> MGSSHHHHHHSSGLVPRGSHMASISKDFTNLLNTLIDGQIGAASRQTEWFNMSPDERTDYIKQVDERLQEMQQSTLSVLAAQHFQMQDNPVSVGDQLQTLQKRRQQMTDVPGTPAINAYKQQLDRDILLYRRQQTAMTHFDSTWRKVLVMLGPDDSKPLNATTLRENAVDKQAKLDTEIKRLEQQLTIQVADSTFSQKYVTLFSELQAYKDVNARYNALLKASATEEAAALGALTKVPQASDDLPVNISLLMMEERPGYIRMNVALVNASTDGRFKDFFLENGRLVVLTDGVLNFSFGTAARSLAWQQQYRLKSEPPSFRSPTYTPIRSVLVKTEFVEKYFANYLVSESTLRGGFKAQLLGNGRKMLLTSVDRKVPNQIGIQVSGQAPNTTITREVPLASALSDLINQNADIASFRTIGLEGFRQSSYHPDRDGLFVNIHELERSVGFAGRQYLLEMPQDNDYLSATPFGVMSVDGDKVSSSHLSKAQTDTLYQYNAAFFEKLEQLRSGGMKASRLFEGSIERTAFVQQLVRLLERNHITPAGVLAPEYPRDNMRDIKGNNLNKVLWEQAFAASVWRSRDNDPLLFRLATRLVKNPAVVKVLQNGYVQSDIAQARELLAPLYEQWRTRAVEAETQRVASANAAQHPSNPKVHVFDQAEVERSLDDKLLILLLTGPQSLEGTDVQLRPMVEAALLSNEGRSLRKQILFHALRPVADSFSKAAAPVNPHAELGVGKIMINNRLNQPDPYLILNTSSEEQAYRDGSYLIKDDKYRSYNQFRP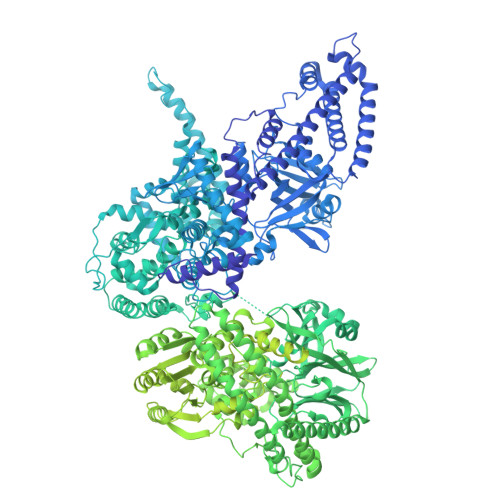DFKNDATRYMNDLDTPFVGGISGTTQTVSNVLTELFGGALSVKQYWQFQMANAAFMIRNGYHSFFETFYVAARYEPEGADSIGKEMLQMFDKYRVEGSKKALQGKLYDGVMARVLPIINQGLSAADEFHPPRFTRIGPRPALLGQAVKDLELKAGLTSVGDGFEPRQGSADIHQFVTDPVLFAKTHTVSAEALVRSGRLPAEGSAQLVKVGSGLYELEYTEQSANDISSSSIPAYFLGYNGPNQANAVPAYVDIPKRTIAGNFLFTGTLSGGSLVVTSLDANTFRVYHDGRVNSSLLYDNVVMAVDYKDYQIAGTAEGLAAAYMQYVNHEWQLVLQRQEYQRDGQMLRLRLRDDEEPLSIQVADSQVVERNQAQFVAYREQIHQQLKKVATQFEVSISGVSDGVYTEGEFSPDHPAIAAWAKLCAEVYDRINADTKQLVDKRNKLYENRRNTIRRDLINQQIKQLNITLEYYKAQYDTVLREAGFVEQSWLWQQIKAKNGSAAVVRIDDTAIQGGGKQRTDSVGERYAISEAYQRGARGTGFSDGLRNFREIEIPGVDDKMSALEMKRLFLEGKLTSEQQGALSGRITETSRAEYIDKVLRQTAVFSEDFHDAGSVFDRLVPQDFYLSLVGDRSGGRAYPLVRAMTVALASGGEAGINSLVQKLFFASADPQAGSSTLLRNSLIKLHSNVEAVQASTELGQFGLSEVVSRLAATTGTSMFALNTQNHSMMVGSTVTTEGRRYYFYDPNVGIFAFDNTKSLSRAMEQHLVGRRLAVHYGSFGSKSAPAFNLIEIDTGKMAEVPVGNGLNVADLTRFEELSSVIGQRRQVEQVMSAQERITEDLQLSTALQAFDAEQWGARFEAASTRLAQEHQLDSRWLPIIATTEEQGEGRYRVQFINRDQPEQTRWLDTDDSTFVEFRRFVDEHMSVLNEHFTLESGRMRPRGGVGEAAPVDGLNAGFAVQALIQWFSDKNRHDAANGMASPDLATALKVHSYLNFVQMVHGGVQDVIKVTALVRTALRGEVVAAQTSFKEFALSLGHTVNEGVGVLFGGAMIGLDAYELAHAENDVQKAVFGTQLAFDSASFVTGAAGIGAGLVGASTAGAVLGGAGVILGGLAVGFTALAQAFGAVAEDAKAVGRYFDTVDKAYKGNGYRYDNEKQVLVPLAGAVIKTLDLSKNQIDFDSQYIYRTHSGSTGSGKINYFFWVGDFPRMVHDRGQAIEVRSGIGYKDVSRPLEHGDSNVVILPGTPKSYISYEYMLLPGATTRHDAGFDVIRRLEEDKRFDYDFYIFPGEETIRRIHHEYVDTPIEVVLDQRNRQLVAPELPKELHGFLCYEIKGAGGEYLIGLNEGAKVNLTSDVASTWIIDSSQLASDSISVSKDQLLVGEKGKEVVVKLYLAQNSQVLVVNGKGEVRKVDFTSLTAQVISEDASKWQVPGQQIEQHLSDLAKAHQLHGQYVVVENYRHQGRDVGRAFYDVTKDRMLFTDTTNEQAKRAQLGAVMGDYAYFYDADNAVAWRVDIATGQVDAQFEPWFNQNAGHISRFWQEGDVVYLARRYRLKEREAELGYRIIGDRMELVSAVGDDALLQLSARIGRHGDELEAILQGYRSNSTQRGTLMYTLGARLIQPTSAALVTVFGVDAAGVPHRYWIRTSDGTLIKPNLAPPADQTLHFEAHEQTRSAWQIPADLVLAGSMPLLGGKEVFFFYSKEQKTLFRQEGPGQEVLDANQPSALRVTTPALTNVINLNGHLVVVTEDGRVARLDALGQLSYAAVNEHWLKGRIHWWQDLTSVTDGRATLAVFGVKDTDGKSLLPVWYHNGQVVVASAALQDKHPQFLGFEVDGSSARLFEPASGKLYRQPAMTADALAAAFGTDEVLEASAQLPAANELEPELHLKAAEQVDAGLRLTTVKGEILLRTHDGKLQLVAVDKDWQQDNLVRLSQALAEVAGQWRVKGVLTLQGDDTQGWFDVGSGQVFSIGGIPATDNLRFIGIAVGKKGAYVYNPTDQMLYQVKESGAQKLNHYADVERIGSSLLLQDGGKGDLSPMLIAGVDSVVLHGGAGSDTYRLSQTMWSYYRTVVIDNDDPNQVLDRLIILAVDAEKIFVSRHEDDLMLTDSVNGTVLVIRKVFGSQAVTHRHLQIDLEGSSSVISVDHLVKGFTR>[2x]GSGAVAVLAESELGSEAQRERRKRILDAT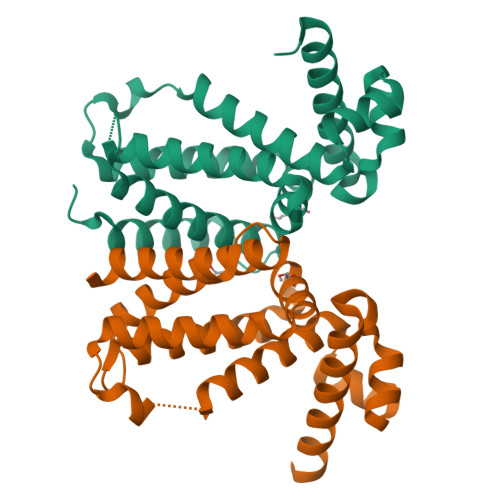MAIASKGGYEAVQMRAVADRADVAVGTLYRYFPSKVHLLVSALGREFSRIDAKTDRSAVAGATPFQRLNFMVGKLNRAMQRNPLLTEAMTRAYVFADASAASEVDQVEKLIDSMFARAMANGEPTEDQYHIARVISDVWLSNLLAWLTRRASATDVSKRLDLAVRLLIGDQDSA> MREYKLVVLGSGGVGKSALTVQFVQGIFVEKYDPTIEDSYRKQVEVDCQQCMLEILD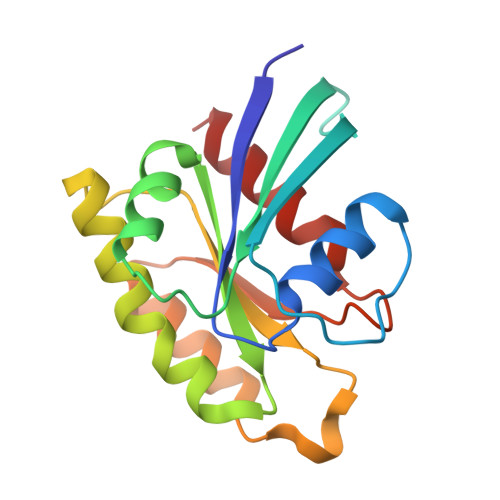TAGTEQFTAMRDLYMKNGQGFALVYSITAQSTFNDLQDLREQILRVKDTEDVPMILVGNKCDLEDERVVGKEQGQNLARQWCNCAFLESSAKSKINVNEIFYDLVRQINR> AAAAAFAAFAG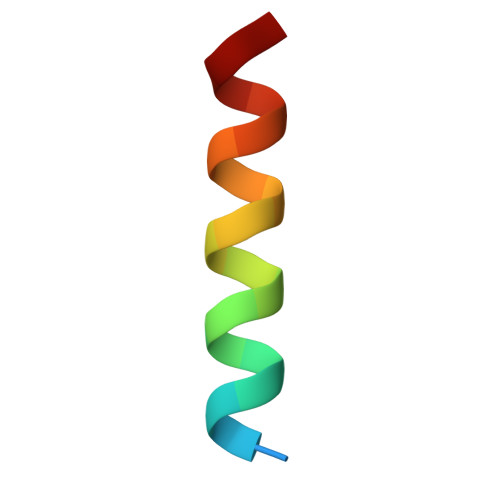FAFAAFAAAG> IVGGQECKDGECPWQALLINEENEGFCGGTILSEFYILTAAHCLYQAKRFKVRVGDRNTEQEEG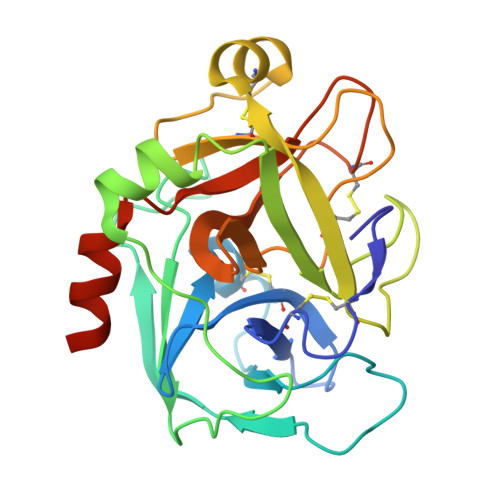GEAVHEVEVVIKHNRFTKETYDFDIAVLRLKTPITFRMNVAPACLPERDWAESTLMTQKTGIVSGFGRTHEKGEQSTRLKMLEVPYVDRNSCKLSSSFIITQNMFCAGYDTKQEDACQGDSGGPHVTRFKDTYFVTGIVSWGEGCARKGKYGIYTKVTAFLKWIDRSMKTRGLPKAK>[2x]MEKKKKLILFNFD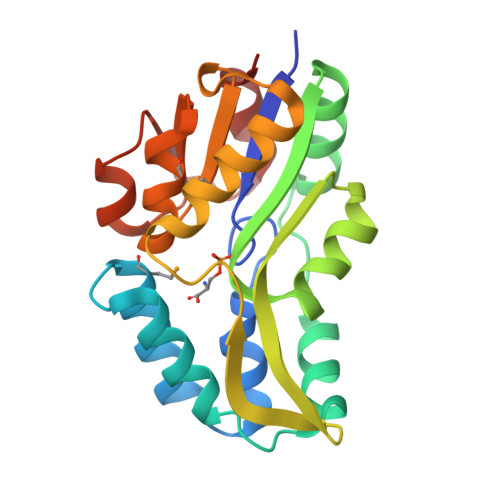STLVNNETIDEIAREAGVEEEVKKITKEAMEGKLNFEQSLRKRVSLLKDLPIEKVEKAIKRITPTEGAEETIKELKNRGYVVAVVSGGFDIAVNKIKEKLGLDYAFANRLIVKDGKLTGDVEGEVLKENAKGEILEKIAKIEGINLEDTVAVGDGANDISMFKKAGLKIAFCAKPILKEKADICIEKRDLREILKYIK>[2x]GAMALNIITVTLNMEKYNFLGISIVGQSNERGDGGIYIGSIMKGG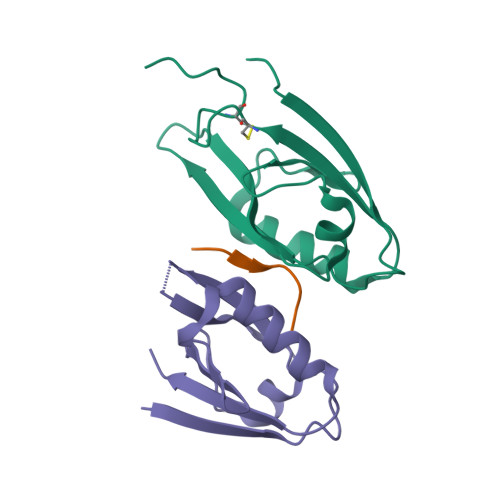AVAADGRIEPGDMLLQVNEINFENMSNDDAVRVLREIVHKPGPITLTVAKCWDPSPRGCFTLPRSE;> SEFFVDVM> EDQKLSDFHADMGGCESCHADGSPSADGAYEFEQCQSCHGSLAEMDAVHKPHDGALMCADCHAPHDMNVGQKPTCDSCHD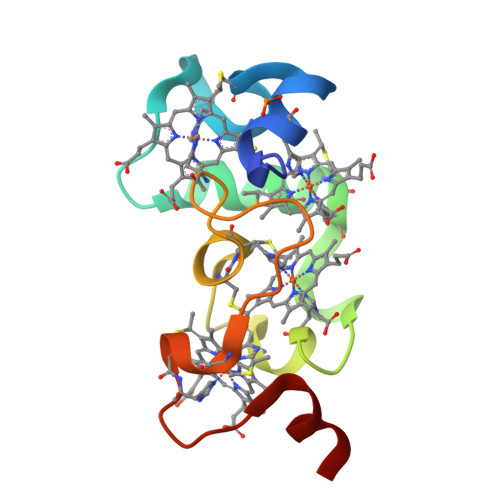DGRTSDSVLK> MAKKTSGRGKLPPGPTPLPVIGNILQIGIKDISKSLTNLSKVYGPVFTLYFGLKPIVVLHGYEAVKEALIDLGEEFSGRGIFPLAERANRGFGIVFSNGKKWKEIRRFSLMTLRNFGMGKRSIEDRVQEEARCLVEELRKTKASPCDPTFILGCAPCNVICSIIFHKRFDYKDQQFLNLMEKLNENIKILSSPWIQICNNFSPIIDYFPGTHNKLLKNVAFMKSYILEKVKEHQESMDMNNPQDFIDCFLMKMEKEKHNQPSEFTIESLENTAVDLFGAGTETTSTTLRYALLLLLKHPEVTAKVQEEIERVIGRNR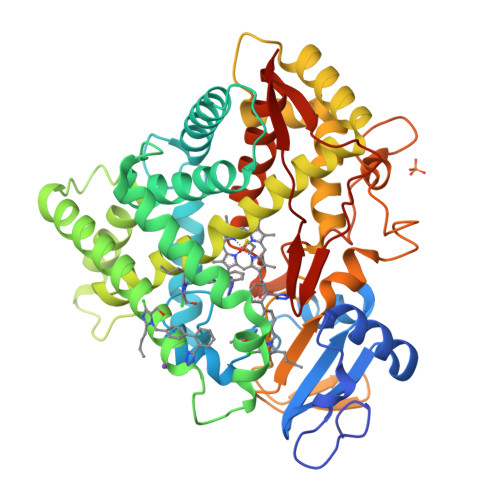SPCMQDRSHMPYTDAVVHEVQRYIDLLPTSLPHAVTCDIKFRNYLIPKGTTILISLTSVLHDNKEFPNPEMFDPHHFLDEGGNFKKSKYFMPFSAGKRICVGEALAGMELFLFLTSILQNFNLKSLVDPKNLDTTPVVNGFTSVPPFYQLCFIPIHHHH> MGRSSILFLLKLMKIMDVQQQQEAMSSEDRFQELVDSLKPRTAHQYKTYYTKYIQWCQLNQIIPTPEDNSVNSVPYKDLPISAELIHWFLLDTLITDDKPGEKREETEDLDEEEENSFKIATLKKIIGSLNFLSKLCKVHENPNANIDTKYLESVTKLHTHWIDSQKAITTNETNNTNTQVLCPPLLKVSLNLWNPETNHLSEKFFKTCSEKLRFLVDFQLRSYLNLSFEERSKIRFGSLKLGKRDRDAIIYHKVTHSAEKKDTPGHHQLLALLPQDCPFICPQTTLAAYLYLRFYGIPSVSKGDGFPNLNADENGSLLQDIPILRGKSLTTYPREETFSNYYTTVFRYCHLPYKRREYFNKCNLVYPTWDEDTFRTFFNEENHGNWLEQPEAFAFPDKIPFDFKKIMNFKSPYTSYSTNAKKDPFPPPKDLLVQIFPEIDEYKRHD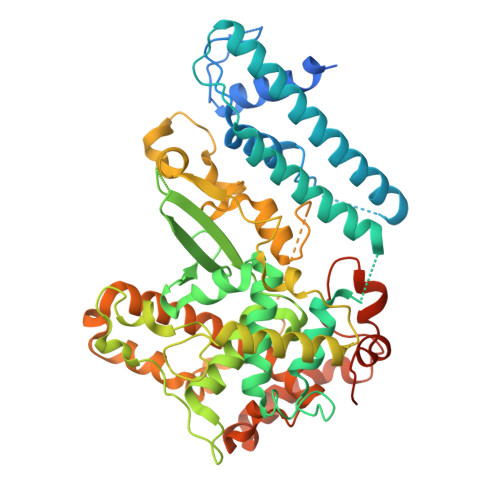YEGLSQNSRDFLDLMEVLRERFLSNLPWIYKFFPNHDIFQDPIFGNSDFQSYFNDKTIHSKGSPILSFDILPGFNKIYKNKTNFYSLLIERPSQLTFASSHNPDTHPWSHPQFEK>[3x]GSKGSRIELGDVTPHNIKQLKRLNQVIFPVSYNDKFYKDVLEVGELAKLAYFNDI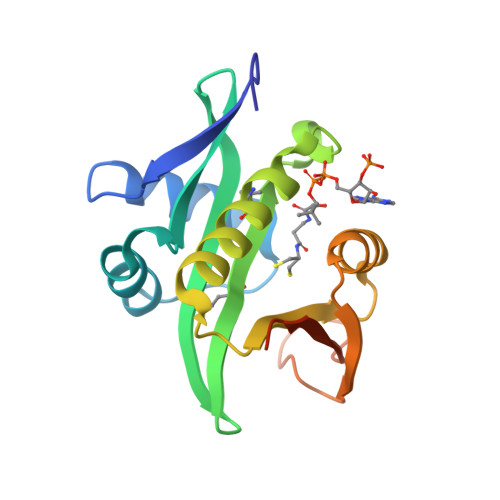AVGAVCCRVDHSQNQKRLYIMTLGCLAPYRRLGIGTKMLNHVLNICEKDGTFDNIYLHVQISNESAIDFYRKFGFEIIETKKNYYKRIEPADAHVLQKNLKVPSGQNADVQKTDN The henipaviruses possess an attachment (G) and a fusion (F) glycoprotein which together work in concert to mediate the virus attachment and entry process, but the precise triggering mechanism of paramyxovirus fusion has yet to be defined in detail. The henipavirus G glycoproteins have a type-II transmembrane topology, containing a short N-terminal cytoplasmic tail and a long C-terminal extracellular globular head. Distinct from most other members within the subfamily Paramyxovirinae, the henipavirus attachment glycoprotein does not hemagglutinate and neither binds to sialic acid, nor retains neuraminidase activity, and instead binds cell surface protein receptors. Recently, ephrin-B2 and ephrin-B3 were identified as the functional receptors for both HeV and NiV.

The high-resolution structures described here, including both HeV-G alone (2.2 Å) and in complex with ephrin-B2 (2.7 Å), combined with structure-based mutagenesis, reveal new insights into the molecular mechanisms governing the initial steps of henipavirus entry into host cells and into the paramyxovirus entry mechanism in general. The HeV-G globular head domain (174–602) was expressed using the baculovirus/insect-cell system as described in the Materials and Methods. The structures reported here indicate that the HeV-G head domain dimer is dissociated upon ephrin binding.

>[2x]YRPISQGVSDLVGLPNQICLQKTTSTILKPRLISYTLPINTREGVCITDPLLAVDNGFFAYSHLEKIGSCTRGIAKQRIIGVGEVLDRGDKVPSMFMTNVWTPPNPSTIHHCSSTYHEDFYYTLCAVSHVGDPILNSTSWTESLSLIRLAVRPKSDSGDYNQKYIAITKVERGKYDKVMPYGPSGIKQGDTLYFPAVGFLPRTEFQYNDSNCPIIHCKYSKAENCRLSMGVNSKSHYILRSGLLKYNLSLGGDIILQFIEIADNRLTIGSPSKIYNSLGQPVFYQASYSWDTMIKLGDVDTVDPLRVQWRNNSVISRPGQSQCPRFNVCPEVCWEGTYNDAFLIDRLNWVSAGVYLNSNQTAENPVFAVFKDNEILYQVPLAEDDTNAQKTITDCFLLENVIWCISLVEIYDTGDSVIRPKLFAVKIPAQCSESGRGLVPR> MAFEAYPPEVNSANIYAGPGPDSMLAAARAWRSLDVEMTAVQRSFNRTLLSLMDAWAGPVVMQLMEA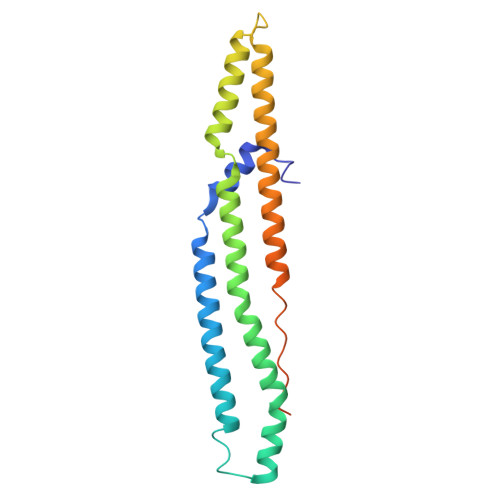AKPFVRWLTDLCVQLSEVERQIHEIVRAYEWAHHDMVPLAQIYNNRAERQILIDNNALGQFTAQIADLDQEYDDFWDEDGEVMRDYRLRVSDALSKLTPWKAPPPIAHSTVLVAPVSPSTASSRTDTLVPR>SNPLEVQAASMRSASEIVQEMGVGWNLGNTLDAKITNLSYNTSPISFETGWGNPVTTKAMIDKIKNAGFKTIRIPTTWGEHLDGNNKLNEEWVKRVKEVVDYCIADDLYVILNTHHEGNWVIPTYAKESSVTPKLKTLWTQISEAFKDYDDHLIFETLNQPRLEGTPYEWTGGTSESRDVVNKYNAAALESIRKTGGNNLSRAVMMPTYAASGSSTTMNDFKVPDDKNVIASVHAYSPYFFAMDTSSNSVNTWGSSYDKYSLDVELDSYLNTFKSKGVPVVIGQFGSINKNNTSSRAE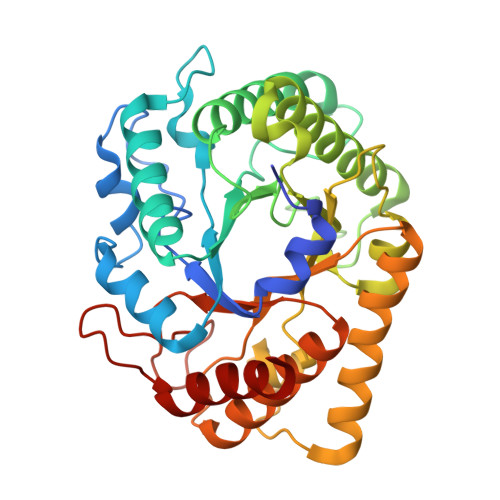LAEYYVTAAQKRGIPCVWWDNNYAETNKGETFGLLNRSTLNWYFSDIKDALIRGYKNVH[2x]>[2x]TNYYYSAVERNNLMRLSQSIPFVPVPPRGEPVTVYRLEESSPSILNNSMSSWSQLGLCAKIEFLSKEEMGGGLRRAVKVLCTWSEHDILKSGHLYIIKSFLPEVINTWSSIYKEDTVLHLCLREIQQQRAAQKLTFAFNQMKPKSIPYSPRFLEVFLLYCHSAGQWFAVEECMTGEFRKYNNNNGDEIIPTNTLEEIMLAFSHWTYEYTRGELLVLDLQGVGENLTDPSVI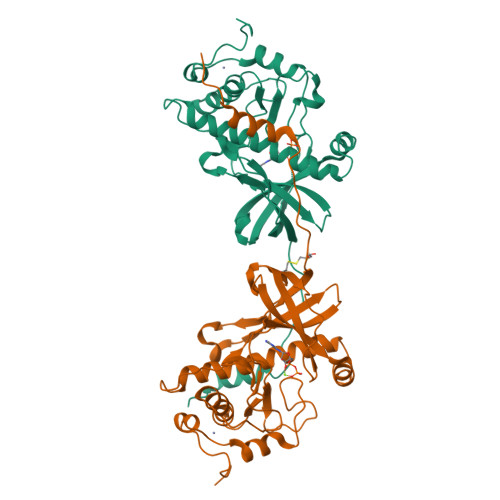KAEEKRSCDMVFGPANLGEDAIKNFRAKHHCNSCCRKLKLPDLKRNDYT>[5x]APQSITELCSEYHNTQIYTINDKILSYTESMAGKREMVIITF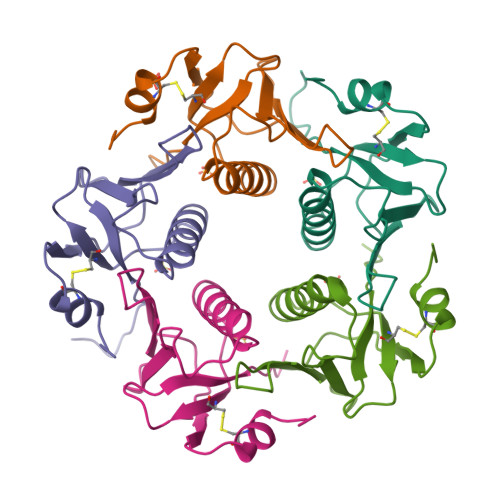KSGATFQVEVPGSQHIDSQKKAIERMKDTLRITYLTETKIDKLCVWNNKTPNSIAAISMEKLYAGAVVNDL> GPLGSSQIPASEQETLVRPKPLLLKLLKSVGAQKDTYTMKEVLFYLGQYIMTKRLYDAAQQHIVYCSNDLLGDL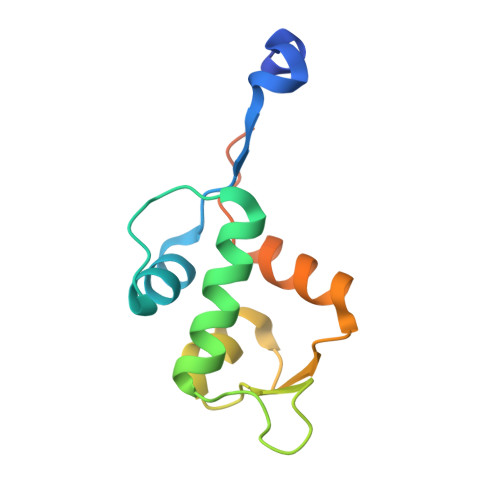FGVPSFSVKEHRKIYTMIYRNLVVVNQQESSDSGTSVSEN>GSKVEDPKDFPSELLSFLSHAVFSNRTLACFAIYTTKEKAALLYKKIMEKYSVTFISRHNSYNHNILFFLTPHRHRVSAINNYAQKLCTFSFLICKGVNKEYLMYSALTRDPFSVIEESLPGGLKEHDFNPESS[2x]

SV40 T-ag is a 708–amino acid protein containing at least three independent functional domains: an N-terminal J domain (amino acids 1–130), a central origin binding domain (obd) (amino acids 131–260), and a C-terminal helicase domain (amino acids 266–625). In the case of SV40, a single virally encoded initiator, large T-antigen (T-ag), can bind the SV40 origin, assemble as a set of two hexameric rings, and cause local distortions (ie, melting) of the DNA. The T-ag obd recognizes the GAGGC-containing duplex DNA at the origin and also binds double-stranded DNA (dsDNA) and ssDNA in a non–sequence-specific manner. In this paper we describe two crystal structures of the SV40 large T-ag obd: one in complex with duplex DNA and one as a dimer in the absence of DNA.

The second crystal structure we report is that of a T-ag obd dimer in the absence of DNA. This structure has been refined to 2.6-Å resolution. The asymmetric unit contains two T-ag obd molecules linked together by a disulfide bond. Although the presence of the disulfide bond is likely an artifact of crystallization, we include it here because it facilitates our description of structural changes associated with DNA binding. Perhaps coincidentally, the obds in this dimer are oriented in a head-to-head fashion and contact one another using the same loops which mediate the inter-obd contacts in the structures of BPV E1. The monomers are related by a pseudo 2-fold symmetry axis with a rotation of 178° between the molecules. The dimer interface contains a mixture of hydrophobic and hydrophilic interactions and buries a surface area of approximately 740 Å2. The T-ag obd–obd interface is nearly symmetric with almost identical residues (18 total) from each monomer contributing atoms to the interaction surface. These residues are from helix αB (Glu166, Leu170, Lys173, and Lys174), residues at the end of helix αC, and residues from the B3 loop (amino acids 213–218). In addition, the cysteine residue bridging the two obds (Cys216) is completely conserved across the Polyoma virus family, and the C216G mutation in T-ag has been shown to be defective in unwinding closed circular DNA. The two obds from the DNA complex structure have the A1 loop in one orientation (flipped “down”), while the three obds crystallized in the absence of DNA have the A1 loop in another conformation (flipped “up”).>[4x]MIRKAFVMQVNPD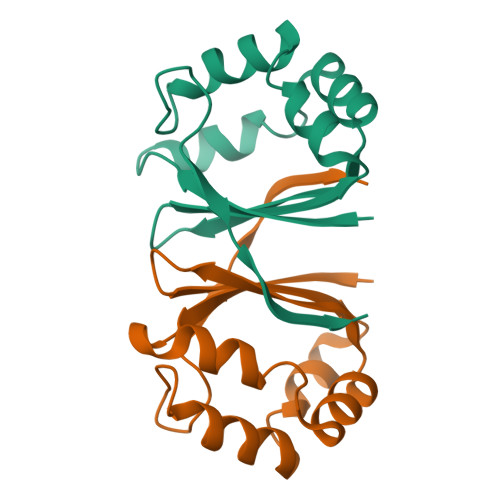AHEEYQRRHNPIWPELEAVLKSHGAHNYAIYLDKARNLLFAMVEIESEERWNAVASTDVCQRWWKYMTDVMPANPDNSPVSSELQEVFYLP>MWFGEFGGQYVPETLVGPLKELEKAYKRFKDDEEFNRQLNYYLKTWAGRPTPLYYAKRLTEKIGGAKVYLKREDLVHGGAHKTNNAIGQALLAKLMGKTRLIAETGAGQHGVATAMAGALLGMKVDIYMGAEDVERQKMNVFRMKLLGANVIPVNSGSRTLKDAINEALRDWVATFEYTHYLIGSVVGPHPYPTIVRDFQSVIGREAKAQILEAEGQLPDVIVACVGGGSNAMGIFYPFVNDKKVKLVGVEAGGKGLESGKHSASLNAGQVGVSHGMLSYFLQDEEGQIKPSHSIAPGLDYPGVGPEHAYLKKIQRAEYVAVTDEE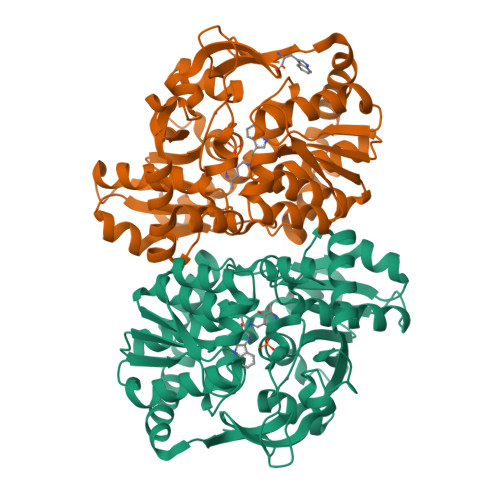ALKAFHELSRTEGIIPALESAHAVAYAMKLAKEMSRDEIIIVNLSGRGDKDLDIVLKASGNVLEHHHHHH[4x]>GAGRHPPVVLVPGDLGNQLEAKLDKPTVVHYLCSKKTESYFTIWLNLELLLPVIIDCWIDNIRLVYNKTSRATQFPDGVDVRVPGFGKTFSLEFLDPSKSSVGSYFHTMVESLVGWGYTRGEDVRGAPYDWRRAPNENGPYFLALREMIEEMYQLYGGPVVLVAHSMGNMYTLYFLQRQPQAWKDKYIRAFVSLGAPWGGVAKTLRVLASGDNNRIPVIGPLKIREQQRSAVSTSWLLPYNYTWSPEKVFVQTPTINYTLRDYRKFFQDIGFEDGWLMRQDTEGLVEATMPPGVQLHCLYGTGVPTPDSFYYESFPDRDPKICFGDGDGTVNLKSALQCQAWQSRQEHQVLLQELPG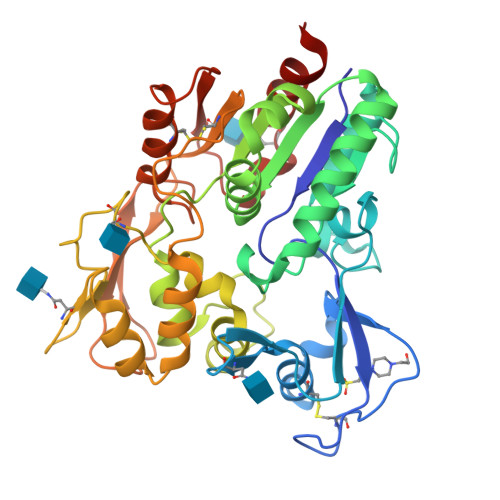SEHIEMLANATTLAYLKRVLLGP[2x]> GMNANQFLKAVSQLQGWRECAFLLALAERSFPNYALFADAVGLKTGGKMRQLLDLAWDMLQKDVADAAIPQLLSKLETLCPNVDEYDAYGVYPAFDFCQLLEQALLNRLNPNKHRATEASQLATRTVMDFVEMSE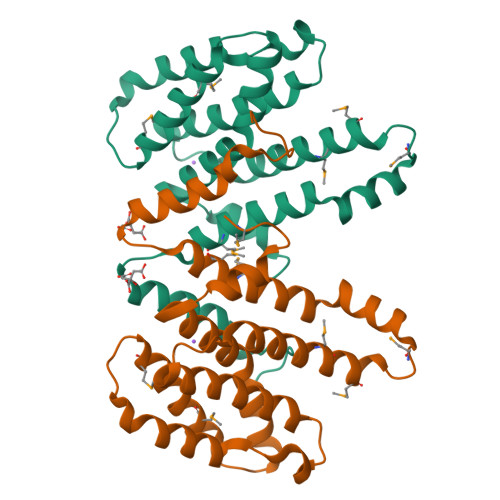GEGMDENELVRVFEHHPLLKDDKLFQRDTVMALYYYRTPKEAFLAELRAGAANDGVSNLGISLEG> ATKAARK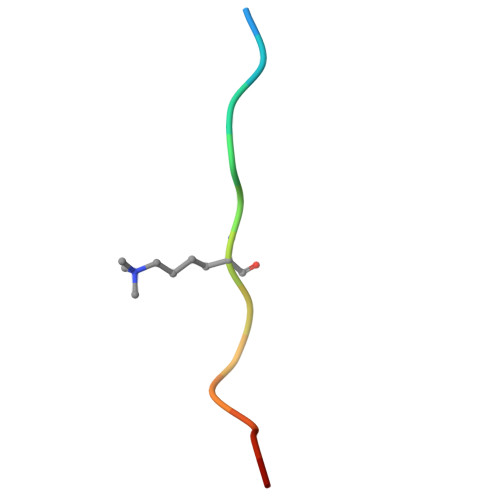SAPATGW> AAN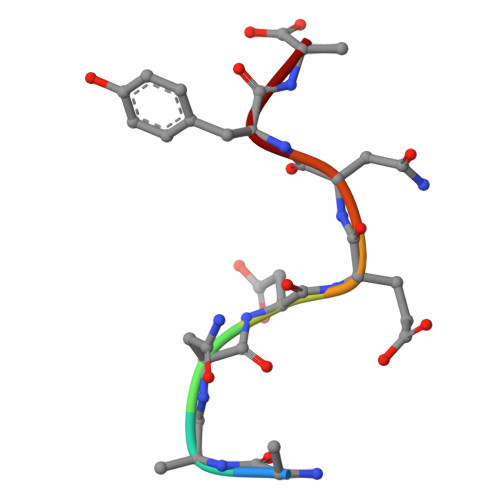DENYA> A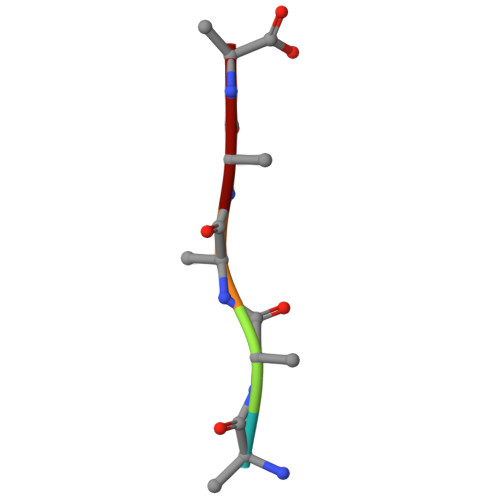AAAA> DRVTTQTAGNTAINTQSSLGVLCAYVEDPTKSDPPSSSTDQPTTTFTAIDRWYTGRLNSWTKAVKTFSFQAVPLPGAFLSRQGGLNGGAFTATLHRHFLMKCGWQVQVQCNLTQFHQGALLVAMVPETTLDVKPDGKAKSLQELNEEQWVEMSDDYRTGKNMPFQSLGTYYRPPNWTWGPNFINPYQVTVFPHQILNARTSTSVDINVPY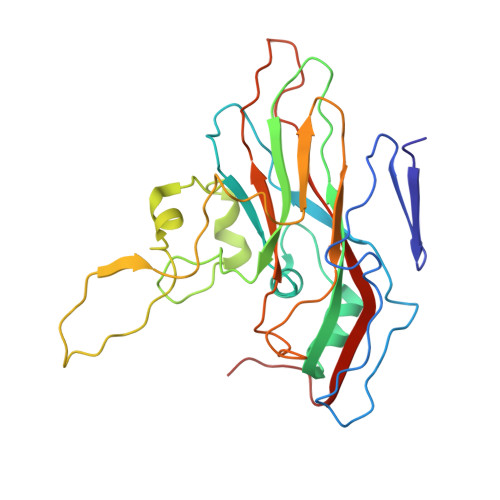IGETPTQSSETQNSWTLLVMVLVPLDYKEGATTDPEITFSVRPTSPYFNGLRNRYTAG> AKTTIIAGSAEAPQGSDIQVPVKIENADKVGSINLILSYP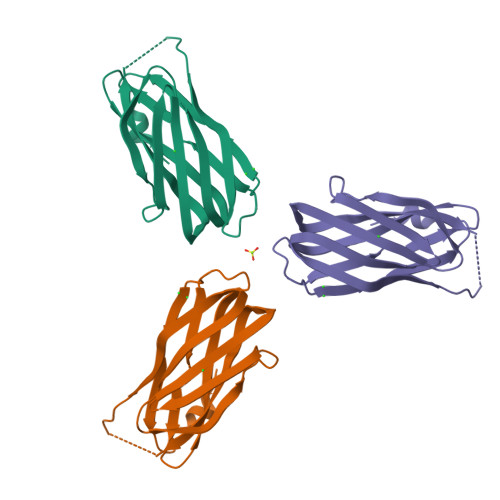NVLEVEDVLQGSLTQNSLFDYQVEGNQIKVGIADSNGISGDGSLFYVKFRVTGNEKAEQAENVKGKLRGLGQQLSEITLRNSHALTLQGIEIYDIDGNSVKVATINGTFRIVSQEEAHHHHHH>MGHHHHHHMKSGRGKKPTRTLVMTSMPSEKQNVVIQVVDKLKGFSIAPDVCETTTHVLSGKPLRTLNVLLGIARGCWVLSYDWVLWSLELGHWISEEPFELSHHFPAAPLCRSECHLSAGPYRGTLFADQPAMFVSPASSPPVAKLCELVHLCGGRVSQVPRQASIVIGPYSGKKKATVKYLSEKWVLDSITQHKVCAPENYLLSQ[2x];>[2x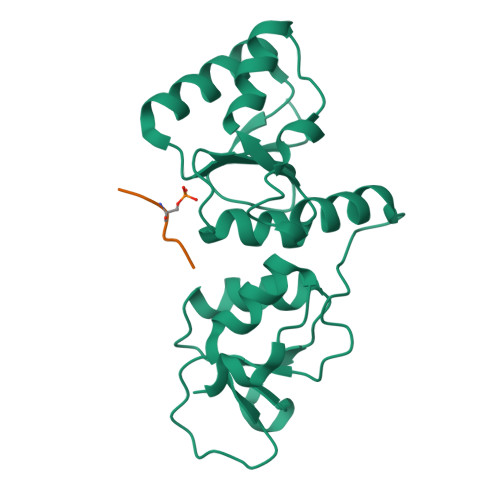]KKATQASQEY One especially common junction element is the kink-turn (k-turn). k-turns are elements in double-stranded RNA that introduce a tight kink into the helical axis, with an included angle close to 50°. A standard k-turn comprises a three-nucleotide bulge followed by successive G•A and A•G trans G(sugar edge)•A(Hoogsteen edge) basepairs. k-turns are commonly-occurring motifs that introduce sharp kinks into duplex RNA, thereby facilitating tertiary contacts. Both the folding and conformation of k-turns are determined by their local sequence. k-turns fall into two conformational classes, called N3 and N1, that differ in the pattern of hydrogen bonding in the core. We show here that this is determined by the basepair adjacent to the critical G•A pairs.

The exceptional N1 structure is Kt-7 observed in the Haloarcula marismortui ribosomal 50S subunit. However, we have shown previously that in other environments, this k-turn (abbreviated here to HmKt-7) adopts the N3 structure. In the course of our studies of k-turns we have determined numerous structures of HmKt-7 removed from the ribosomal context including three new structures reported here, all of which are N3 structures. Moreover, the various structures, with resolutions in the range 1.7 to 3.1 Å, have been determined in five different space groups, encompassing hexagonal, tetragonal and orthorhombic symmetries. Several include multiple molecules within the asymmetric unit and altogether there are 17 independent structures, all of which are unambiguously in the N3 conformation, and all in a closely similar conformation with a small RMSD values. Thus it is clear that the N1 conformation adopted by HmKt-7 in the ribosome is the single exception. In the ribosome the k-turn mediates an important tertiary interaction, and is bound by the L24 protein, and it is likely that these factors force the conformation against its intrinsic nature.

>UGGGGAGCCGAAAGGCGAAGAACC[8x]> XAATSRPERVWPDGVIPFVIGGNFTGSQRAVFRQAMRHWEKHTCVTFL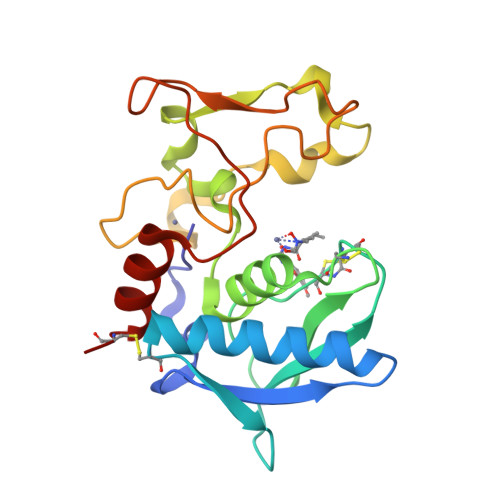ERTDEDSYIVFTYRPCGCCSYVGRRGGGPQAISIGKNCDKFGIVVHELGHVVGFWHEHTRPDRDRHVSIVRENIQPGQEYNFLKMEPQEVESLGETYDFDSIMHYARNTFSRGIFLDTIVPKYEVNGVKPPIGQRTRLSKGDIAQARKLYKCP N-(1-methylethyl)-3-[(3-prop-2-en-1-ylbiphenyl-4-yl)oxy]propan-1-amine 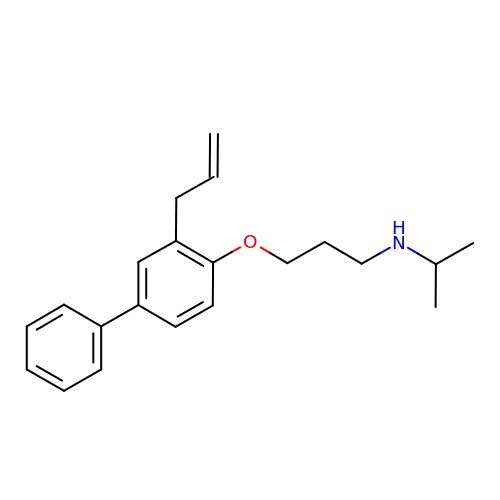| C21 H27 N O | CKIDETHAWPUGOQ-UHFFFAOYSA-N> GREEIFQVALH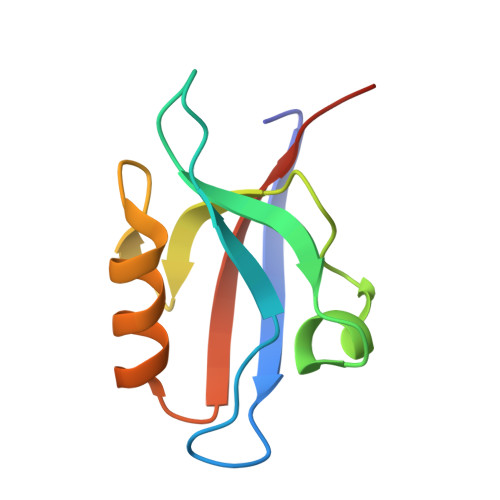KRDSGEQLGIKLVRRTDEPGVFILDLLEGGLAAQDGRLSSNDRVLAINGHDLKYGTPELAAQIIQASGERVNLTIARPGKPQP> QQKPVVKTAQNLAEVNGPETLIGPGAKEGTVPTDLDQETGLARLELLGKLEGIDVFDTKPLDSSRKGTMKDPIIIESYDDYRYVGCTGSPAGSHTIMWLKPTVNEVARCWECGSVYKLNPVGVPNDD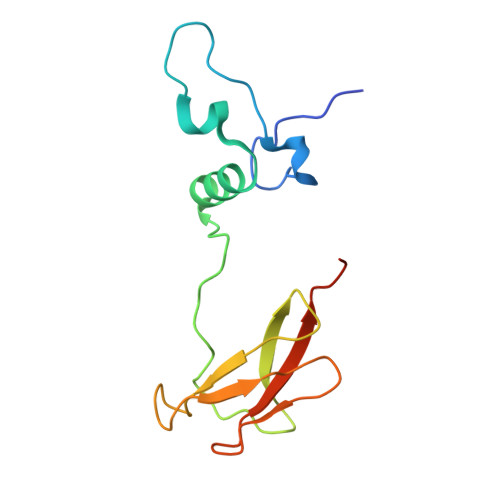HHH4-METHYL-3-(9-OXO-1,8-DIAZA-TRICYCLO[10.6.1.0(13,18)]NONADECA-12(19),13(18),15,17-TETRAENE-10-CARBAMOYL)PENTA-METHYLSULFONEDIIMINE | C25 H39 N5 O2 S | 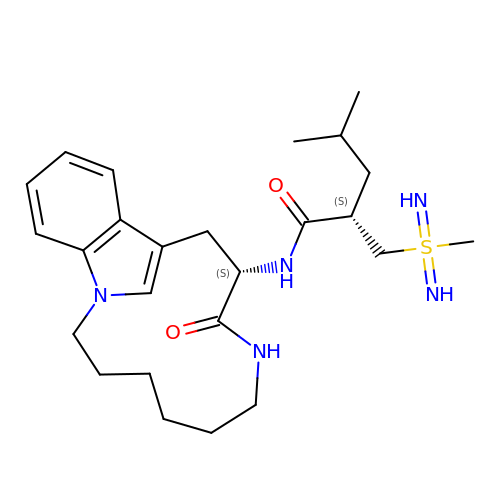MQEMTMGYPYUQLH-IRLDBZIGSA-N> MNIQILQEQANTLRFLSADMVQKANSGHPGAPLGLADILSVLSYHLKHNPKNPTWLNRDRLVFSGGHASALLYSFLHLSGYDLSLEDLKNFRQLHSKTPGHPEISTLGVEIATGPLGQGVANAVGFAMAAKKAQNLLGSDLIDHKIYCLCGDGDLQEGISYEACSLAGLHKLDNFILIYDSNNISIEGDVGLAFNENVKMRFEAQGFEVLSINGHDYEEINKALEQAKKSTKPCLIIAKTTIAKGAGELEGSHKSHGAPLGEEVIKKAKEQAGFDPNISFHIPQASKIRFESAVELGDLEEAKWKDKLEKSAKKELLERLLNPDFNKIAYPDFKGKDLATRDSNGEILNVLAKNLEGFLGGSADLGPSNKTELHSMGDFVEGKNIHFGIREHAMAAINNAFARYGIFLPFSATFFIFSEYLKPAARIAALMKIKHFFIFTHDS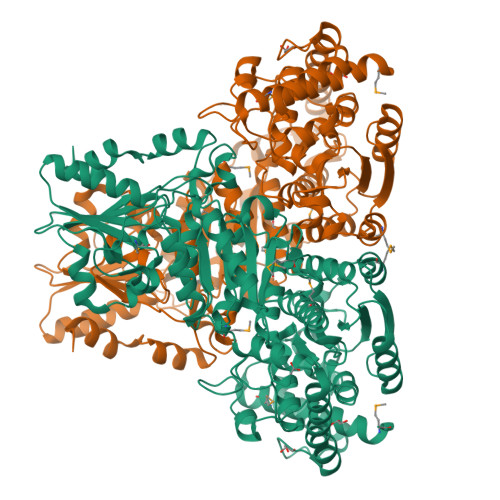IGVGEDGPTHQPIEQLSTFRAMPNFLTFRPADGVENVKAWQIALNADIPSAFVLSRQKLKALNEPVFGDVKNGAYLLKESKEAKFTLLASGSEVWLCLESANELEKQGFACNVVSMPCFELFEKQDKAYQERLLKGEVIGVEAAHSNELYKFCHKVYGIESFGESGKDKDVFERFGFSVSKLVNFILSK6-(2-(5-((2-methoxyethyl)(methyl)amino)pyridin-3-yl)ethyl)-4-methylpyridin-2-amine | C17 H24 N4 O | 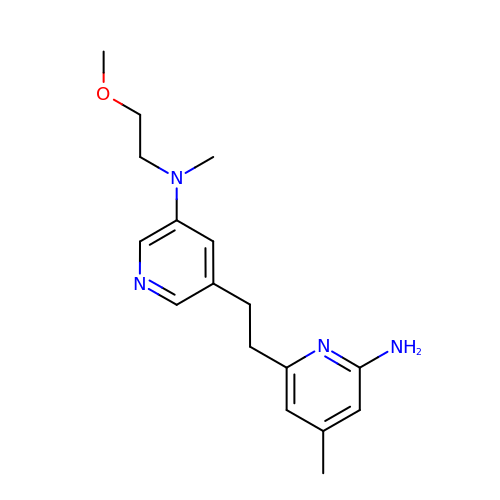PDIACSYIIWCGFI-UHFFFAOYSA-N>[10x]GSAPADNAADARPVDVSVSIFINKIYGVNTLEQTYKVDGYIVAQWTGKPRKTPGDKPLIVENTQIERWINNGLWVPALEFINVVGSPDTGNKRLMLFPDGRVIYNARFLGSFSNDMDFRLFPFDRQQFVLELEPFSYNNQQL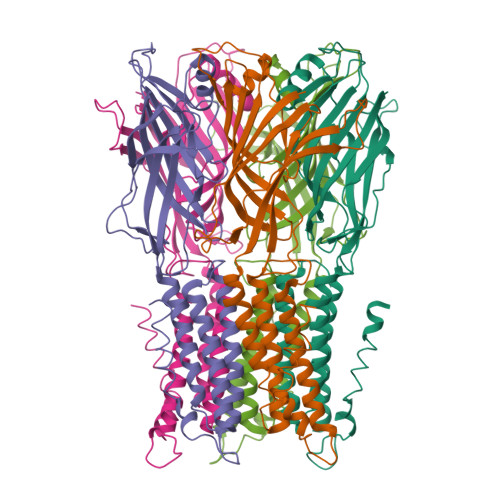RFSDIQVYTENIDNEEIDEWWIRGKASTHISDIRYDHLSSVQPNQNEFSRITVRIDAVRNPSYYLWSFILPLGLIIAASWSVFWLESFSERLQTSFTLMSTVVAYALYTSNILPRLPYTTVIDQMIIAGYGSIFAAILLIIFAHHRQANGVEDDLLIQRCRLAFPLGFLAIGCVLVIRGITL>MRSRRVDVMDVMNRLILAMDLMNRDDALRVTGEVREYIDTVKIGYPLVLSEGMDIIAEFRKRFGCRIIADFKVADIPETNEKICRATFKAGADAIIVHGFPGADSVRACLNVAEEMGREVFLLTEMAHPGAEMFIQGAADEIARMGVDLGVKNYVGPSTRPERLSRLREIIGQDS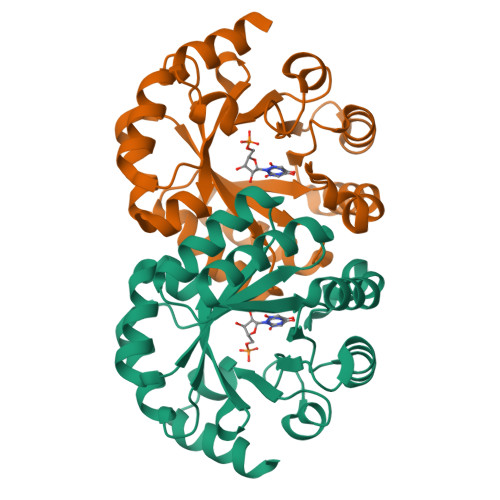FLISPGVGAQGGDPGETLRFADAIIVGRSIYLADNPAAAAAGIIESIKDLLIPEDPAANKARKEAELAAATA[2x]>[2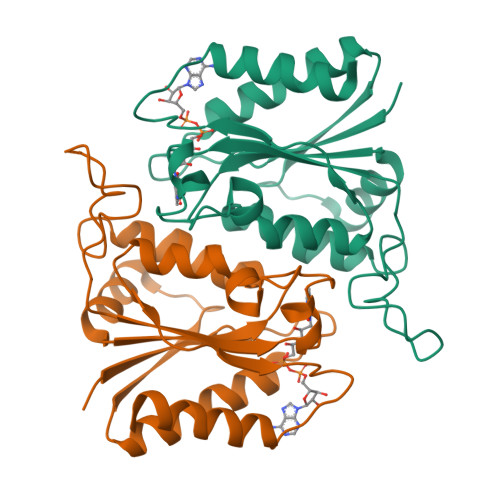x]MGSSHHHHHHGSSNILIINGAKKFAHSNGQLNDTLTEVADGTLRDLGHDVRIVRADSDYDVKAEVQNFLWADVVIWQMPGWWMGAPWTVKKYIDDVFTEGHGTLYASDGRTRKDPSKKYGSGGLVQGKKYMLSLTWNAPMEAFTEKDQFFHGVGVDGVYLPFHKANQFLGMEPLPTFIANDVIKMPDVPRYTEEYRKHLVEIFG>[2x]GPLMDTTIDGFADSYEISSTSFVATDNTDSSIVYLAAEQVLTGPDVSALQLLSNSFESVFDSPDDFYSDAKLVLSDGREVSFHRCVLSARSSFFKSALAAAKKEKDSNNTAAVKLELKEIAKDYEVGFDSVVTVLAYVYSSRVRPPPKGVSECADENCCHVACRPAVDFMLEVLYLAFIFKIPELITLYQRHLLDVVDKVVIEDTLVILKLANICGKACMKLLDRCKEIIVKSNVDMVSLEKSLPEELVKEIIDRRKELGLEVPKVKKHVSNVHKALDSDDIELVKLLLKEDHTNLDDACALHFAVAYCNVKTATDLLKLDLADVNHRNPRGYTVLHVAAMRKEPQLILSLLEKGASASEATLEGRTALMIAKQATMAVECNNIPEQCKHSLKGRLCVEI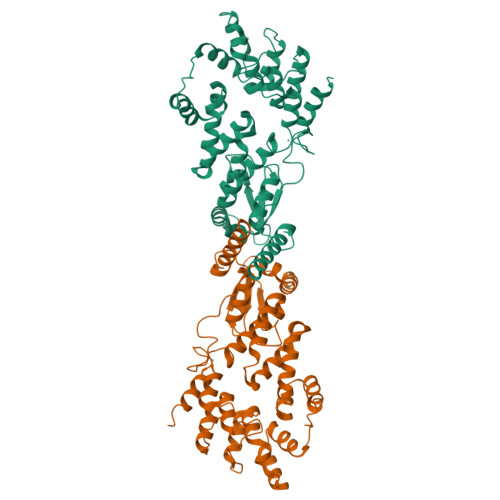LEQEDKREQIPRDVPPSFAVAADELKMTLLDLENRVALAQRLFPTEAQAAMEIAEMKGTCEFIVTSLEPDRLTGTKRTSPGVKIAPFRILEEHQSRLKALSKTVELGKRFFPRCSAVLDQIMNCEDLTQLACGEDDTAEKRLQKKQRYMEIQETLKKAFSEDNLELGNSSLTDSTSSTSKSTGGKRSNRKLSHRRRGGWSHPQFEK> GHIMSMTPE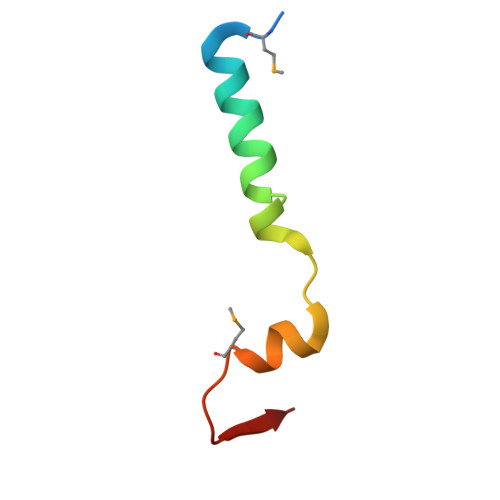QLQAWRWEREIDERNRPLSDEELDAMFPEGYKVL>[4x]MNRESFAAGERLVSPAYVRQGCEARRSHEHLIRLLLEKGKCPENGWDESTLELFLHELAIMDSNNFLGNCGVGEREGRVASALVARRHYRFIHGIGRSGDISAVQPKAAGSSLLNKITNSLVLDIIKLAGVHTVANCFVVPMATGMSLTLCFLTLRHKRPKAKYIIWPRIDQKSCFK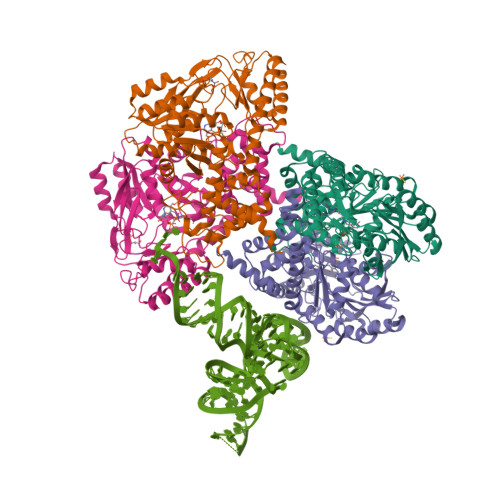SMITAGFEPVVIENVLEGDELRTDLKAVEAKVQELGPDCILCIHSTTSCFAPRVPDRLEELAVICANYDIPHIVNNAYGVQSSKCMHLIQQGARVGRIDAFVQSLDKNFMVPVGGAIIAGFNDSFIQEISKMYPGRASASPSLDVLITLLSLGSNGYKKLLKERKEMFSYLSNQIKKLSEAYNERLLHTPHNPISLAMTLKTLDEHRDKAVTQLGSMLFTRQVSGARVVPLGSMQTVSGYTFRGFMSHTNNYPCAYLNAASAIGMKMQDVDLFIKRLDRCLKAVRKERSKESDDNYDKTEDVDIEEMALKLDNVLLDTYQDASS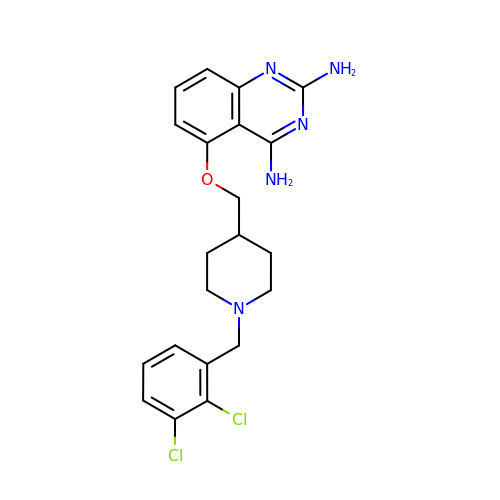5-{[1-(2,3-dichlorobenzyl)piperidin-4-yl]methoxy}quinazoline-2,4-diamine | C21 H23 Cl2 N5 O | XVLUVRFYGVJKGJ-UHFFFAOYSA-N~{N}-[(~{Z},2~{S},3~{R})-1,3-bis(oxidanyl)heptadec-4-en-2-yl]dodecanamide 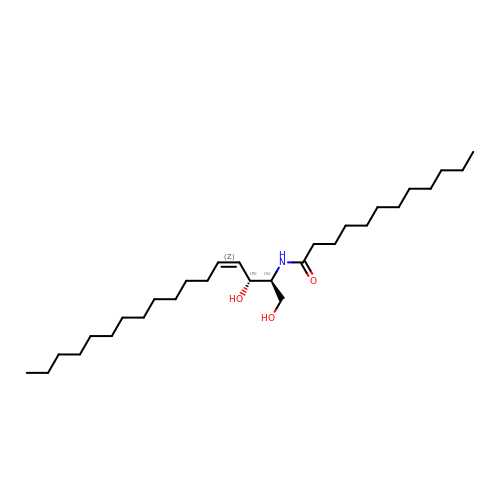| C29 H57 N O3 | CUYUYRQLXJHPEB-UWJMOZLHSA-N>[4x]METWVLGRRDVAEVVAAVGRDELMRRIIDRLTGGLAEIGRGERHLSPLRGGLERSEPVPGIWEWMPHREPGDHITLKTVGYSPANPARFGLPTILGTVARYDDTTGALTALMDGV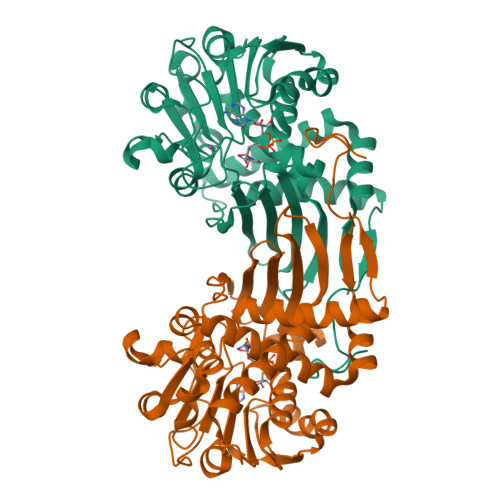LLTALRTGAASAVASRLLARPDSHTLGLIGTGAQAVTQLHALSLVLPLQRALVWDTDPAHRESFARRAAFTGVSVEIAEPARIAAEADVISTATSVAVGQGPVLPDTGVREHLHINAVGADLVGKTELPLGLLERAFVTADHPEQALREGECQQLSADRLGPQLAHLCADPAAAAGRQDTLSVFDSTGFAFEDALAMEVFLEAAAERDLGIRVGIEHHPGDALDPYALQ>GHMSHTILLVQPTKRPEGRTYADYESVNECMEGVCKMYEEH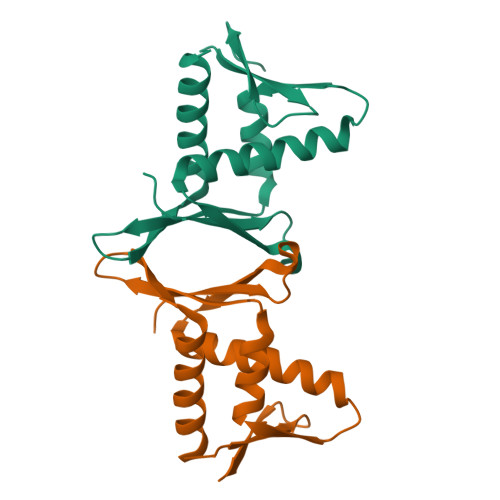LKRMNPNSPSITYDISQLFDFIDDLADLSCLVYRADTQTYQPYNKDWIKEKIYVLLRRQAQQAGKGSSGSSGSSGSSGSSGSSGSSPGVWGAGGSLKVTILQSSDSRAFSTVPLTPV[4x]The PIWI-clade Argonautes (PIWIs) bind 24–31-nt PIWI-interacting RNAs (piRNAs) to form piRNA-induced silencing complexes, which silence transposons and maintain genome integrity in animal gonads. In contrast, Piwi co-transcriptionally silences transposons in the nucleus, by facilitating heterochromatin formation at target transposon loci. The Piwi–piRNA complex interacts with nascent transposon transcripts and essential cofactors, such as the zinc-finger protein Gtsf1/Asterix (Arx)13–15 and the adaptor protein Silencio/Panoramix (Panx). The structure revealed that Piwi consists of four domains (N, PAZ, MID, and PIWI) and three linker regions (L0, L1, and L2), and it can be divided into two lobes (N-PAZ and MID-PIWI).

In this study, we purified the endogenous Piwi–piRNA complex from cultured fly ovarian somatic cells (OSCs), and determined the crystal structure of the Piwi–piRNA complex at 2.9 Å resolution. Indeed, 32P-end labeling of the RNAs revealed that about 26-nt RNAs are associated with Piwi, consistent with previous studies. These results indicated that the purified sample represents the Piwi–piRNA complex core (residues 34–843) lacking the flexible N-terminal region. We observed relatively poor electron densities for the PAZ domain, indicating that the PAZ domain is flexible in the present structure. The resulting model is consistent with the anomalous difference peaks for two putative mercury ions (derived from the crystallization solution), which are located in the vicinities of Cys271 and Cys317. The 5′ end of the bound piRNA is flipped into a pocket between the MID and PIWI domains of Piwi, whereas nucleotides 2–4 of the piRNA adopt an A-form-like conformation with their Watson–Crick edges exposed to the solvent, as in Siwi and hAgo2. The 5′ phosphate group of the piRNA is recognized by the side chains of Tyr551, Lys555, Gln567, and Lys593, and the main-chain amide group of Val568. We observed an anomalous difference density in the vicinity of the 5′ phosphate group, where we modeled a zinc ion derived from the crystallization solution. The zinc ion is coordinated by phosphates 1 and 3 in the piRNA, the side chain of Gln589, and the C-terminal carboxyl group of Leu843. The present structure revealed that Piwi has the DVDK (Asp614/Val653/Asp685/Lys818), rather than DEDH, tetrad in the PIWI domain, and that Val653, corresponding to the glutamate finger, adopts the “unplugged” conformation. A structural comparison between Piwi and Siwi indicated that the structural features, such as the N domain orientation and the metal-dependent piRNA recognition, are conserved among the PIWI-clade Argonautes.

> RGSSSGDPRADPRIEASRERRALEEAPRREGGPTERKPWGDQYDYLNTRPAELVSKKGTDGVPVMLQTNFFRLKTKPEWRIVHYHVEFEPSIENPRVRMGVLSNHANLLGSGYLFDGLQLFTTRKFEQEITVLSGKSKLDIEYKISIKFVGFISCAEPRFLQVLNLILRRSMKGLNLELVGRNLFDPRAKIEIREFKMELWPGYETSIRQHEKDILLGTEITHKVMRTETIYDIMRRCSHNPARHQDEVRVNVLDLIVLTDYNNRTYRINDVDFGQTPKSTFSCKGRDISFVEYYLTKYNIRIRDHNQPLLISKNRDKALKTNASELVVLIPELCRVTGLNAEMRSNFQLMRAMSSYTRMNPKQRTDRLRAFNHRLQNTPESVKVLRDWNMELDKNVTEVQGRIIGQQNIVFHNGKVPAGENADWQRHFRDQRMLTTPSDGLDRWAVIAPQRNSHELRTLLDSLYRAASGMGLRIRSPQEFIIYDDRTGTYVRAMDDCVRSDPKLILCLVPNDNAERYSSIKKRGYVDRAVPTQVVTLKTTKNRSLMSIATKIAIQLNCKLGYTPWMIELPLSGLMTIGFDIAKSTRDRKRAYGALIASMDLQQNSTYFSTVTECSAFDVLANTLWPMIAKALRQYQHEHRKLPSRIVFYRDGVSSGSLKQLFEFEVKDIIEKLKTEYARVQLSPPQLAYIVVTRSMNTRFFLNGQNPPPGTIVDDVITLPERYDFYLVSQQVRQGTVSPTSYNVLYSSMGLSPEKMQKLTYKMCHLYYNWSGTTRVPAVCQYAKKLATLVGTNLHSIPQNALEKKFYYL>MSDKDSKNTPQVPEKLGLSRRGFLGASAVTGAAVAATALGGAVMTRESWAQAVKESKQKIHVGPGELDDYYGFWSGGHQGEVRVLGVPSMRELMRIPVFNVDSATGWGLTNESRHIMGDSAKFLNGDCHHPHISMTDGKYDGKYLFINDKANSRVARIRLDIMKCDKMITVPNVQAIHGLRLQKVPHTKYVFANAEFIIPHPNDGKVFDLQDENSYTMYNAIDAETMEMAFQVIVDGNLDNTDADYTGRFAAATCYNSEKAFDLGGMMRNERDWVVVFDIHAVEAAVKAGDFITLGDSKTPVLDGRKKDGKDSKFTRYVPVPKNPHGCNTSSDGKYFIAAGKLSPTCSMIAIDKLPDLFAGKLADPRDVIVGEPELGLGPLHTTFDGRGNAYTTLFIDSQVVKWNMEEAVRAYKGEKVNYIKQKLDVHYQPGHLHASLCETNEADGKWLVALSKFSKDRFLPVGPLHPENDQLIDISGDEMKLVHDGPTFAEPHDCIMARRDQIKTKKIWDRNDPFFAPTVEMAKKDGINLDTDNKVIRDGNKVRVYMTSMAPAFGVQEFTVKQGDEVTVTITNIDQIEDVSYGFVVVNHGVSMEISPQQTSSITFVADKPGLHWYYCSWFCHALHMEMVGRMMVEPAWSHPQ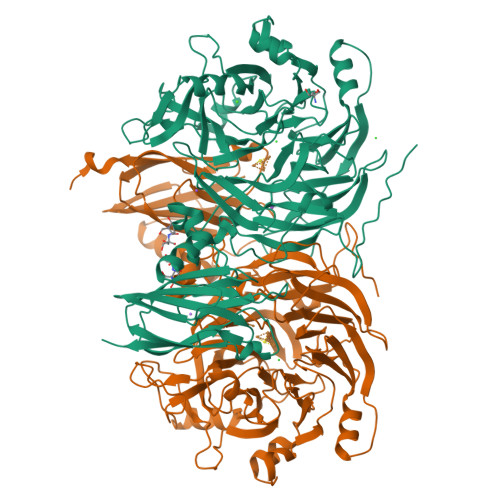FEK[2x]Cytosolic PLA2α (cPLA2α), a Group IV mammalian PLA2 family member, preferentially releases arachidonic acid from PLs in a cytosolic Ca2+-concentration-dependent manner. Arachidonic acid generated by cPLA2α is a precursor of pro-inflammatory eicosanoids, including certain prostaglandins and leukotrienes. Mechanistically, the membrane translocation of cPLA2α is driven primarily by its N–terminal C2-domain rather than its catalytic domain. Complexation of two Ca2+ ions by the C2-domain neutralizes several Asp residues, facilitating protein docking and penetration into the membrane interface region.

However, using purified Gallus gallus (chicken) cPLA2α C2-domain (81% identical and 93% highly conserved sequence relative to human), we obtained crystal complexes with 1,2-dihexanoyl-sn-glycero-3-phosphocholine (DHPC), enabling structure determination at 2.2 Å resolution. Three C2-domain molecules comprise the asymmetric unit and each C2-domain contains one bound DHPC molecule. The C2-domain–DHPC complex exhibits a β-sandwich topology formed by a pair of four-stranded antiparallel β-sheets (one formed by the β4, β1, β8 and β7 strands; the other by the β3, β2, β5 and β6 strands). In contrast to the two bound Ca2+ ions reported in the lipid-free structure, we observed three Ca2+ ions coordinated in the PC-bound structural complex, consistent with the established Ca2+ dependence of membrane interaction by the C2-domain. We found that the Ca1 ion is bound via side-chain interactions with Asp40, Asp43, Asp93 and Asn95 and the main chain carbonyl group of Ala94; whereas Ca4 is bound via interaction with the side chains of Asp40, Asp43 and Asn65 and the main-chain carbonyl group of Thr41. CaPC, which was not observed in two previous lipid-free structures, bridges the C2-domain to DHPC via its phosphoryl group (3.6 Å) and sn-1 carbonyl group (3.2 Å) and also interacts with the Asn65 side-chain (3.1 Å). Although Ca1 does not coordinate with the DHPC molecule, Ca4 does interact with two oxygen atoms of the DHPC phosphoryl group in bifurcated fashion (2.1 and 3.7 Å). The only direct interaction between the phosphoryl group and the C2-domain is a hydrogen bond with the side chain of Asn65 (~3.1 Å). Importantly, the Tyr96 aromatic ring stacks in planar-like fashion with the cationic -N+(CH3)3 group. The DHPC polar headgroup docks with the CBLs, whereas the fatty acid chains are largely exposed to solvent.

>[3x]GSYSHVFTVTVRKATNVTKGAIGDMLDTPDPYVELFIPSAPDCRKRTKHFNNDVNPVWNETFEFILDPNQDNVLEVTLMDANYVMDETLGMATFPISSLKLGEKKEVQLTFNNVTEMTLELSLEVCS> AILHKYMGIFFSTMSSEELLGSLDSFDAREDDIFLVSYPKSGTHWLAEVIERIPDAGITL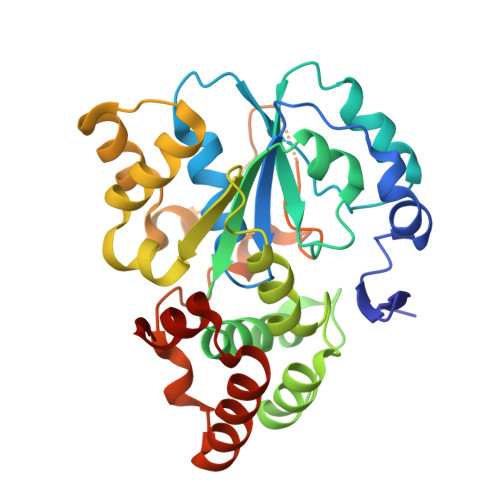TSPIELGDISKFEELKRIPKRRAIPTHLNYEMLPVTVKQKQCKIIYIVRNPKDTAVSMFHYYRDNPNLPSTETWAAFLELFLKGDVVYGSWFDHVLSWEEHKNDKNVLFIFYEEMKKDFVKSLKKITAFLGIDVNDSEMAKIARSTSFSEMKSNAAKENCDPNHVICALTSDRNLVFRKGVVGDWINYFTPKQNRGFDELFTEKMRNSDVGRCLKEYAHSA> XSLSDKDKAAVKLLWSKISKSSDAIGNDALSRMIVVYPQTKTYFAHWPDLSPGSPHVKAHGKTVMGGIALAVSKIDDLRAGLLDLSEQHAYKLRVDPANFKILSHCILVVISMMFPKEFTPEAHVSLD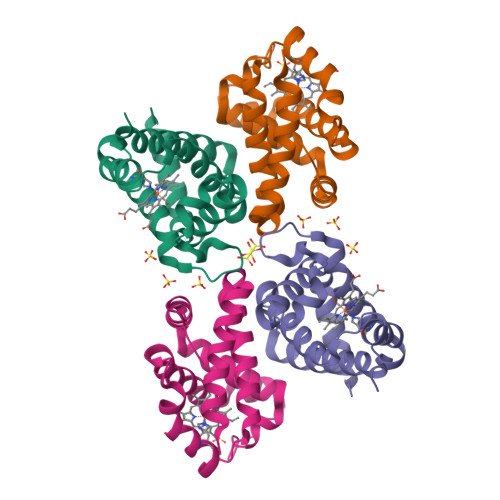KFLSGVSLALSERYR;> VEWTDQERATISSIFGSLDYDDIGPKALSRCLIVYPWTQRHFGSFGNLYNAEAIIGNQKVAAHGIKVLHGLDRAVKNMDNIKEIYAELSILHSEKLHVDPDNFKLLADCLTIVVAAKMGSGFNPGTQATFQKFLAVVVSALGKQ IadD interacts with IadE to form a functional Rieske non-heme dioxygenase, which works in concert with a FMN-type reductase encoded by gene iadC to transform IAA into the biologically inactive 2-oxindole-3-acetic acid (oxIAA), representing a new bacterial pathway for IAA inactivation/degradation. The Rieske non-heme iron dioxygenases, typically composed of α and β subunits that are equivalent to IadD and IadE, respectively, share a conserved α3β3 configuration. IadD features a Rieske domain (residues 44–160) and a catalytic domain (residues 1–43 and 161–437). IadE is a single-domain protein, containing a twisted seven-stranded β-sheet and 3 α-helices, which may mainly serve as a scaffold protein contributing to proper assembly of the oligomeric enzyme complex.

To understand the binding of IAA with IadD, we then determined a 2.6 Å cryo-EM structure of IadD/E complexed with IAA. An overall mushroom-shaped heterohexamer composed of 3 IadE at the “stem” and 3 IadD in the “cap” was resolved. The active site of IadD is located at the interface of IadD subunits, composed of a Rieske [2Fe-2S] cluster from the Rieske domain and a mononuclear iron in the catalytic domain of a neighboring subunit. The [2Fe-2S] is stabilized by contacts with Cys85, His87, Cys106, and His109 and the mononuclear iron coordinates with His216, His221, and Asp377. Adjacent to the mononuclear iron is the IAA-binding pocket lined by polar and hydrophobic residues including Asn210, Leu211, His216, His221, Phe251, His311, Lys322, Arg329, and Tyr362. No profound overall conformational changes were observed for IadD/E after binding of IAA. The side chain of His311 in IadD is relocated to accommodate the binding of IAA. The mononuclear iron and the coordinating residues also move slightly inwards (about 1.6 Å) following the binding of IAA. The resolved IAA-binding pocket of IadD/E is largely superimposed with that of biphenyl in the biphenyl dioxygenase structure, but contains different residues to accommodate the substrate specificity. As anticipated, mutation of residues in the pocket abrogated IAA binding.

>[3x]MAGTEVTRQDLIDFVVNEAHLLDTRRYEEWNALFTDDAFYWVPLVPDQEDGLNHTSHLYEDKLLRELRIERLKSPRAFSQQPPSRCHHLLQVPVVEQFDAEGNRFVLRTGFHYTESQGDELQFYVGTFFHHLTVRDGALRMTLKRVNLLNCDAALPAVQLFI;>[3x]MTSYRDNPDAIRALVQDDRVHRDLYTSQELFELEQEHFFANTWNYVGHESQLPKPGDWISNEIAGRPLIVARHSDGSVRAMMNRCAHKGSRLVNGPCGNTGKFFRCPYHAWTFKTDGSLLAIPLKTGYENTALHECESAKGLTTLRYVRSHRGFIFVKISDAGPDFDDYFGDSLSSIDNMADRSPEGELEIAGGCLRFMHQCNWKMFVENLNDTMHPMVAHESSAGTAKRMWADKPEDEPKPMAVEQFAPFMSDYKFFEDMGIRTYDNGHSFTGVHFSIHSKYKAIPAYDDAMKARYGEAKTAQILGMARHNTVYYPNLTIKGAIQAIRVVKPISADRTLIESWTFRLKGAPPELLQRTTMYNRLINSPFSVVGHDDLQAYRGMQAGLHASGNEWVSLHRNYDPSELKGGEITTGGTNELPMRNQYRAWVQRMTETM> MNQAYVKRHLIGRVVIPKLAVDL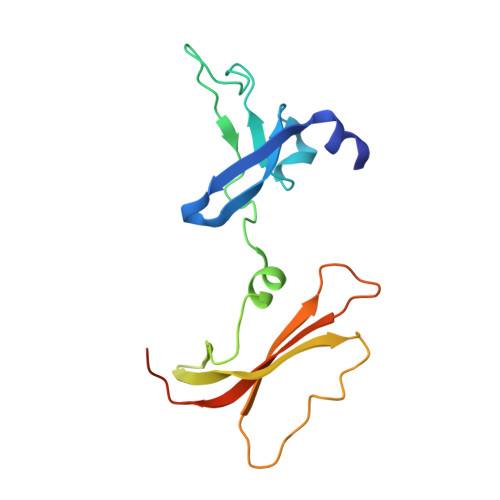PLFDTTNNTLLDQGAVVLPGTSYPRGGKNTHTVVSAHGGLPTKRFFTDLSKLKRGQKFFLQVNGKKMAYQVFRIKTVRPDETQSLRIEPGRDLATLMTCTPYMINSHRLLVTGKRVPYTESLEHHHHHH>YTNSDFVVIKALEDGVNVIGLTRGADTRFHHSEKLDKGEVLIAQFTEHTSAIKVRGKAYIQTMHGVIESEGK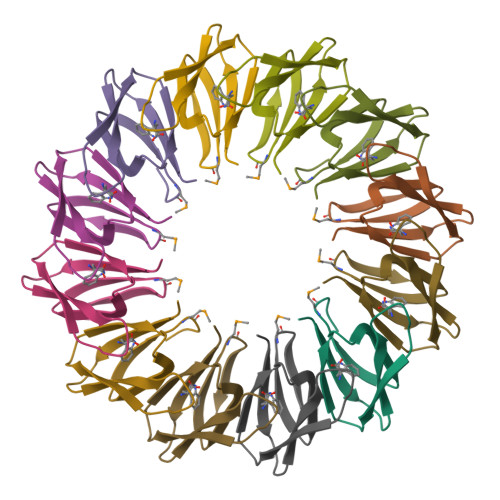KAAAM[3x]Most importantly, the T6SS from the Gram-negative, pathogenic bacterium Pseudomonas aeruginosa was shown to inject at least three different effector molecules (named Tse1, Tse2, and Tse3; Type-6-Secretion-Exported) into the periplasmic space of competing cells. Tse1 was shown to be an amidase that cleaves the γ-D-glutamyl-l-meso-diaminopimelic acid amide bond of crosslinked PG, and Tse3 is a muramidase that cleaves the PG-backbone between the N-acetylmuramic acid and the N-acetylglucosamine moieties. As injection of effector proteins by the T6SS would also cause cell death of siblings, P. aeruginosa co-synthesizes the cognate immunity proteins Tsi1 and Tsi3 (Type-6-Secretion-Immunity) and shuttles them into their periplasmic space to confer resistance. Tse1 adopts the fold of N1pC/P60 papain-like cysteine peptidases, which are widespread among bacteria and of which homologues were identified in eukaryotes, phages, viruses, and archaea.

We crystallized P. aeruginosa Tse1 and obtained excellent data, for which experimental structure factor phases were obtained from a Single-wavelength Anomalous Diffraction (SAD) experiment on selenomethionine-substituted protein crystals. Subsequently, the model was refined against 2.6 Å resolution data. In both structures, four molecules per asymmetric unit were found which were virtually identical to each other. Both models show excellent stereochemistry, with 96% of the residues in the preferred regions of the Ramachandran plot. Since DSB2 was observed in the highly redundant SAD data, collected at the selenium peak, its absence in the native structure is unlikely to be caused by radiation damage. However, once we excluded any reducing agents from the purification procedure of native Tse1 protein and setup crystallization experiments, crystals with similar morphology as observed for selenomethionine-substituted proteins were observed suggesting that in those crystals DSB2 had been formed too. Thus, we argue that DSB2 formation or not is not an experimental artifact. Indeed, it is possible that in cytosolic Tse1 DSB2 is open, and that it closes after transportation into the periplasmic space by T6SS.

>[4x]MDSLDQCIVNACKNSWDKSYLAGTPNKDNCSGFVQSVAAELGVPMPRGNANAMVDGLEQSWTKLASGAEAAQKAAQGFLVIAGLKGRTYGHVAVVISGPLYRQKYPMCWCGSIAGAVGQSQGLKSVGQVWNRTDRDRLNYYVYSLASCSLPRASAAALEHHHHHH>MGHHHHHHHHHHMSKQQIGVVGMAVMGRNLALNIESRGYTVSIFNRSREKTEEVIAENPGKKLVPYYTVKEFVESLETPRRILLMVKAGAGTDAAIDSLKPYLDKGDIIIDGGNTFFQDTIRRNRELSAEGFNFIGTGVSGGEEGALKGPSIMPGGQKEAYELVAPILTKIAAVAEDGEPCVTYIGADGAGHYVKMVHNGIEYGDMQLIAEAYSLLKGGLNLTNEELAQTFTEWNNGELSSYLIDITKDIFTKKDEDGNYLVDVILDEAANKGTGKWTSQSALDLGEPLSLITESVFARYISSLKDQRVAASKVLSGPQAQPAGDKAEFIEKVRRALYLGKIVSY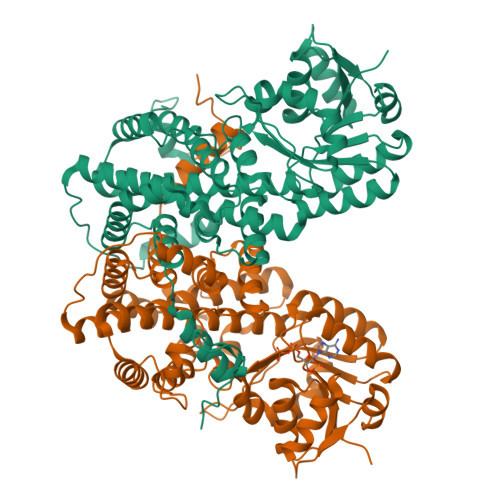AQGFSQLRAASEEYNWDLNYGEIAKIFRAGCIIRAQFLQKITDAYAENPQIANLLLAPYFKQIADDYQQALRDVVAYAVQIGIPVPTFSAAVAYYDSYRAAVLPANLIQAQRDYFGAHTYKRIDKEGVFHTEWLD[2x]> MHLYSSDFPLMMDEKELYEKWMRTVEMLKAEGIIRSKEVERAFLKYPRYLSVEDKYKKYAHIDEPLPIPAGQTVSAPHMVAIMLEIANLKPGMNILEVGTGSGWNAALISEIVKTDVYTIERIPELVEFAKRNLERAGVKNVHVILGDGSKGFPPKAPYDVIIVTAGAPKIPEPLIEQLKIGGKLIIPVGSYHL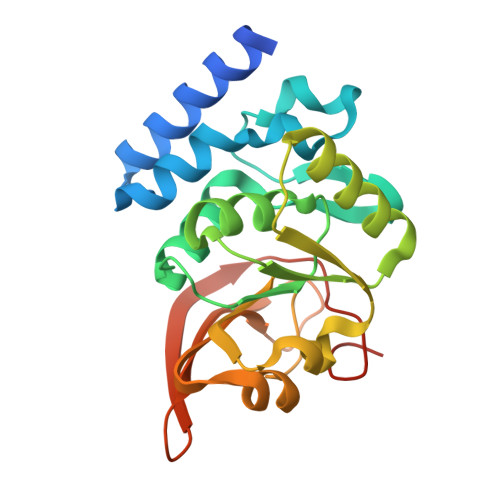WQELLEVRKTKDGIKIKNHGGVAFVPLIGEYGWKEHHHHHH> GHSSSDP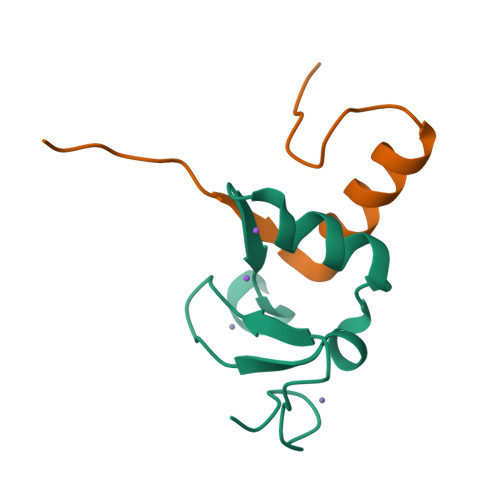VYPCGICTNEVNDDQDAILCEASCQKWFHRICTGMTETAYGLLTAEASAVWGCDTCMA;> AMAAKVVYVFSTEMANKAAEAVLKGQVETIVSFHI> MASMSETSCDLQATNYIRGCQSKTYDGKIFPGKGGEKQWICKDTIIHGDTNGACIPPRTQNLCVGELWDKSYGGRSNIKQDTKELLKEKIKNAI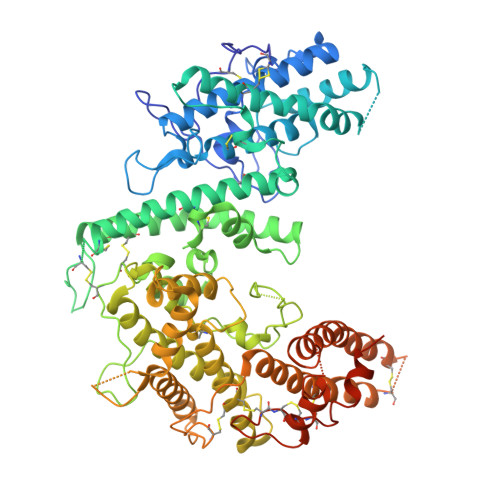HKETELLYEYHDTGTAIISKNDKKGQKGKNDPNGLPKGFCHAVQRSFIDYKNMILGTSVNIYEHIGKLQEDIKKIIEKGTPQQKDKIGGVGSSTENVNAWWKGIEREMWDAVRCAITKINKKNNNGIFNGDECGVSPPTGNDEDQSVSWFKEWGEQFCIERLRYEQNIREACTINGKNEKKCINSKSGQGDKIQGACKRKCEKYKKYISEKKQEWDKQKTKYENKYVGKSASDLLKENYPECISANFDFIFNDNIEYKTYYPYGDYSSICSCEQVKYYKYNNAEKKNNKLLCYEKDNDMTWSKKYIKKLENGRSLEGVYVPPRRQQLCLYELFPIIIKNEEGMEKAKEELLETLQIVAEREAYYLWKQYNPTGKGIDDANKKACCAIRGSFYDLEDIIKGNDLVHDEYTKYIDSKLNEIFGSSDTNDIDTKRARTDWWENEAITNGPDRKTIRQLVWDAMQSGVRYAVEEKNENFPLCMGVEHIGIAKPQFIRWLEEWTNEFCEKYTKYFEDMKSKCDPPKRADTCGDNSNIECKKACANYANWLNPKRIEWNGMSNYYNKIYRKSNKESEGGKDYSMIMAPTVIDYLNKRCHGEINGNYICCSCKNIGAYQTTSGTVNKKLQKKETECEEEKGPLDLMNEVLNKMHHHHHH(3S,5R)-5-{[(4-methylphenyl)sulfonyl]amino}-N-(9H-xanthen-9-ylmethyl)piperidine-3-carboxamide 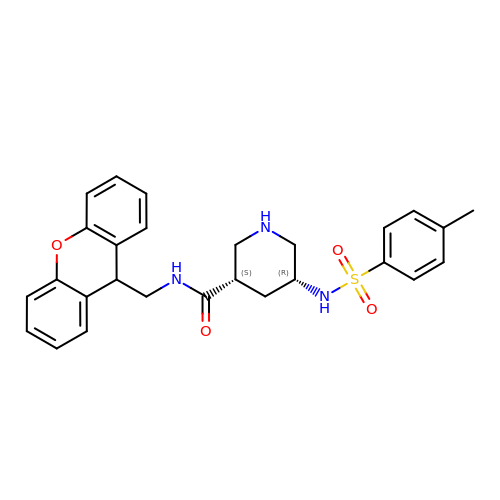| C27 H29 N3 O4 S | SOEKUZSTSXYGKH-VQTJNVASSA-N> RELASKDPGAVDAKP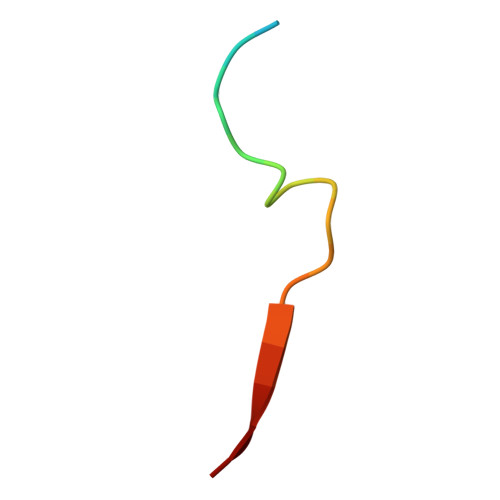LVVEI>[2x]MKELFQKIWQNELQFLNFDAKFQDKSKLDTAECAIILSVNKDNYERYFLLKEFQELCKKIDLRVDIFSMQNAQICILNLFKSGFISKQDLLKALKILEKISKNTEIFDFILQEKVQSIDQKALFQNDFKELNTINLELQKLSFDENLKSRLQKTLEKFQNLEFNIAITGVMNAGKSSLLNALLKEDFLGVSNIPETANLTVLSYGKSEEAKIYFWDKKEWQNILESSHFNADLKEFIDKLDKSVNIEDFIKDKPLIQNIALCELKNFSSAKNKISALIKKIEIKSHLEFLKNNISIVDTPGLDDVVVQREIVTNEYLRESDFLIHLMNASQSLTQKDADFLVHCLLNSRLSKFLIVLTKADLLSKKDLEEVIVYTKESLKSRLVDLDENLVEKIDFLCVSAKMASDFYKGLASKESLQKSGMQEFENYLFNELYAGEKSKIALRAYKKELHLELKNILSEYEMQNRLIKENKQGVSEENQKLLLELQKQNTLLKEAQDEISNSIAKLKNIDSGIDNLVLLLAKKLKERLIDEFKYLKNNAQKLNLSRILNIVDITTKDGINDILREIKFENIKKIEELKTNLSLKYDFLKDDFDNGFEGFKDGISKNIDSIFQSEKFALLRLKIEKLSNLKSDLYELETNLDTVIFDTFKEFKMSEILNSLNINGAFFEFLNDKLKHYEKNQKSKLESLEKVLQSLKNQDANILNSFEENLEKIEKLKQLEMGLLNADKLHH;>[2x]GSHMQINLLNDFIKAYENTYSVSFDDSFKGRIQELCKELNEPFMHASYALENELKELVFSLDKNVNIAIIGQFSSGKSSLLNLILGRDCLPTGVVPVTFKPTFLRYAKEYFLRVEFEDGSDIITNIEKLAFYTDQRNEVKQAKSLHIFAPIPLLEKITLVDTPGLNANENDTLTTLDELKNIHGAIWLSLIDNAGKKSEEDAIKANLELLGENSICVLNQKDKLSAEELDNVLNYAKSVFLKYFNELIAISCKEAKDEQSYEKSNFQSLLDFLTQLDTTVLKEKFVKRKILNLCEILEDENQLFVGIFDRLLNQFQSYEKHLLLAYENFLKEIEILNHQILEQLKSISERISSEIFASVKEKDAYFYKESKGFLKKDLYTRYDYKAPYISSDDAFLAMFYNSDVMSKEFKKIKNELYKSFEEIKMKLKDFINILEREILLFKAEFSNIQKDHIFQSDKNFSELRAFCNASDEYFLKDFKELLFKSILELDLFFEKLNLKAFTNYENATKLSLAFFSRKINESRVLYELDSSEFVLFYPKKSEIYERVLNELNVYEFETLLINKPILTKIAKNFLEQSQNLIQEKNKFLDLKKAELQKRRAQILNVRESIKEDHH

Here we structurally and biochemically characterise the DLP pair from Campylobacter jejuni. The respective proteins, here called Cj-DLP1 (84.5 kDa) and Cj-DLP2 (71.2 kDa), were cloned, expressed and purified. Both DLPs are monomeric in solution and form a stable heterotypic tetramer, termed Cj-DLP1/2tetramer, with 2:2 stoichiometry when mixed. The tetramer is dominated by a 2-fold symmetry where Cj-DLP2 with its symmetry mate (termed Cj-DLP2α and Cj-DLP2β) form a central back-to-back cis dimer flanked on each side by Cj-DLP1 (termed Cj-DLP1α and Cj-DLP1β). Combined with GTPase activity and lipid binding, we present a mechanism for how the tetramer tethers and bridges distantly opposing membranes.

Crystals of Cj-DLP1/2tetramer bound to GDP and GDP·AlF4¯ were also obtained in the same P212121 space group as for the apo state. For both, the overall model is essentially identical to apo except for the coordination of GDP within the nucleotide binding pockets. Within the GDP·AlF4¯ crystal, no density for the AlF4¯ moiety was observed. Based on the similarity between the GDP and GDP·AlF4¯ electron densities, it is understood that the GDP·AlF4¯ structure reported here is likely representative of the GDP conformation. Cj-DLP1 has a canonical BDLP1-like fold augmented with an N-terminal 119 amino acid globular domain that nestles between the neck and G-domains. For Cj-DLP2, hinge 2 exists in the closed position so that the GTPase domain (G-domain) nucleotide-binding pocket is oriented orthogonal to the neck-trunk long axis. For the back-to-back cis Cj-DLP2 dimer, the dimerisation interface extends along each symmetry mate so that the GTPase, neck and trunk domains contribute to a substantial buried surface area of 5969 Å2. However, the presence of assembly-stimulated nucleotide turnover, which requires both Cj-DLP1 and Cj-DLP2 GTPase domains to be active, strongly suggests nucleotide binding triggers hetero G-dimer formation.> GSARENEMDENLEQ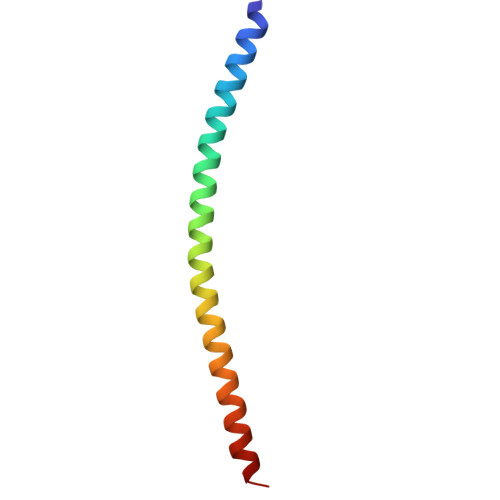VSGIIGNLRHMALDMGNEIDTQNRQIDRIMEKADSNKTRIDEANQRATKML> DSGFSFG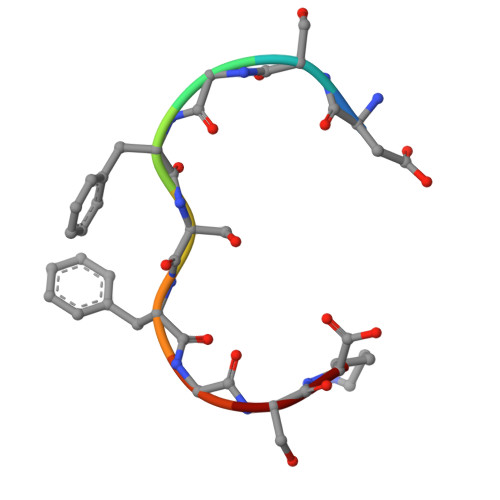SK> MNFSEQQLINWSRPVSTTEDLKCQNAITQITAALRAKF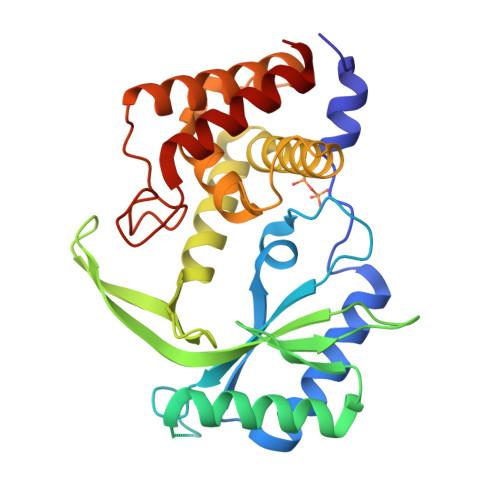GNRVTIFLQGSYRNNTNVRQNSDVDIVMRYDDAFYPDLQRLSESDKAIYNAQRTYSGYNFDELKADTEEALRNVFTTSVERKNKCIQVNGNSNRITADVIPCFVLKRFSTLQSVEAEGIKFYSDDNKEIISFPEQHYSNGTEKTNQTYRLYKRMVRILKVVNYRLIDDGEIADNLVSSFFIECLVYNVPNNQFISGNYTQTLRNVIVKIYEDMKNNADYTEVNRLFWLFSNRSPRTRQDALGFMQKCWNYLGYQ>MASEKHFKYVILGGGVAAGYAAREFAKQGVKPGELAIISKEAVAPYERPALSKGYLFPQNAARLPGFHVCVGSGGERQLPEWYSEKGIELILSTEIVKADLSTKTLTSAAGATFTYEILIIATGSSVIKLTDFGTQGADSNNILYLREIDDADKLVAAIQAKKGGKAVVVGGGYIGLELSAALKINDFDVTMVFPEPWCMPRLFTADIAAFYEAYYTNKGVKVLKGTLAVGFDANANGDVTAVKLKDGKVLEADIVVVGVGGRPLTTLFKGQV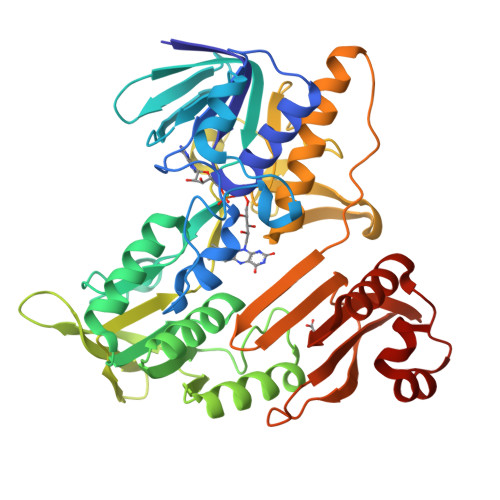AEEKGGIKTDAFFETSVPGVYAIGDVATFPLKMYNELRRVEHVDHSRKSAEQAVKAIKGKESGESVPEYDYLPYFYSRSFDLGWQFYGDNVGETILFGDSDPTSSKPKFGSYWIKDGKVFGAFLEGGSPDENNAIAKVAKTQPPVASIEELKKEGLQFASKI[4x]>[5x]QEEGEDNGGEDNKKLRGALSSAIL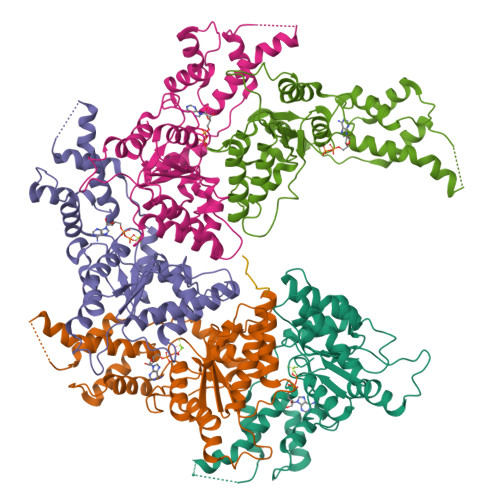SEKPNVKWEDVAGLEGAKEALKEAVILPVKFPHLFKGNRKPTSGILLYGPPGTGKSYLAKAVATEANSTFFSVSSSDLVSKWMGESEKLVKQLFAMARENKPSIIFIDEVDALTGTRGEGESEASRRIKTELLVQMNGVGNDSQGVLVLGATNIPWQLDSAIRRRFERRIYIPLPDLAARTTMFEINVGDTPCVLTKEDYRTLGAMTEGYSGSDIAVVVKDALMQPIRKIQSATHFKDVSTEDDETRKLTPCSPGDDGAIEMSWTDIEADELKEPDLTIKDFLKAIKSTRPTVNEDDLLKQEQFTRDFGQEGN;> XDEIVNKVLX>MAKKTSSKGKLPPGPTPLPIIGNMLQIDVKDICKSFTNFSKVYGPVFTVYFGMNPIVVFHGYEAVKEALIDNGEEFSGRGNSPISQRITKGLGIISSNGKRWKEIRRFSLTTLRNFGMGKRSIEDRVQEEAHCLVEELRKTKASPCDPTFILGCAPCNVICSVVFQKRFDYKDQNFLTLMKRFNENFRILNSPWIQVCNNFPLLIDCFPGTHNKVLKNVALTRSYIREKVKEHQASLDVNNPRDFIDCFLIKMEQEKDNQKSEFNIENLVGTVADLFVAGTETTSTTLRYGLLLLLKHPEVTAKVQEEIDHVIGRHRSPCMQDRSHMPYTDAVVHEIQRYSDLVPTGVPHAVTTDTKFRNYLIPKGTTIMALLTSVLHDDKEFPNPNIFDPGHFLDKNGNFKKSDYFMPFSAGKRICAGEGLARMELFLFLTTILQNFNLKSVDDLKNLNTTAVTKGIVSLPPSYQICFIPVHHHH[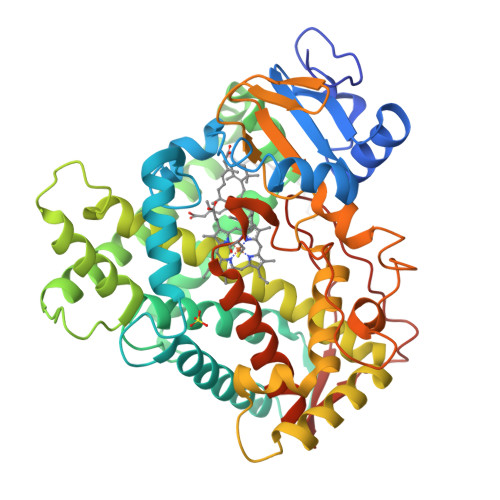2x]> MGVALGATRVIYPAGQKQEQLAVTNNDENSTYLIQSWVENADGVKDGRFIVTPPLFAMKGKKE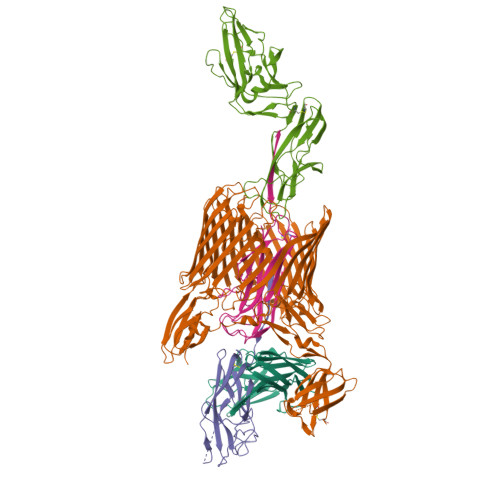NTLRILDATNNQLPQDRESLFWMNVKAIPSMDKSKLTENTLQLAIISRIKLYYRPAKLALPPDQAAEKLRFRRSANSLTLINPTPYYLTVTELNAGTRVLENALVPPMGESTVKLPSDAGSNITYRTINDYGALTPKMTGVME;> DLYFNPRFLADDPQAVADLSRFENGQELPPGTYRVDIYLNNGYMATRDVTFNTGDSEQGIVPCLTRAQLASMGLNTASVAGMNLLADDACVPLTTMVQDATAHLDVGQQRLNLTIPQAFMSNRARGYIPPELWDPGINAGLLNYNFSGNSVQNRIGGNSHYAYLNLQSGLNIGAWRLRDNTTWSYNSSDRSSGSKNKWQHINTWLERDIIPLRSRLTLGDGYTQGDIFDGINFRGAQLASDDNMLPDSQRGFAPVIHGIARGTAQVTIKQNGYDIYNSTVPPGPFTINDIYAAGNSGDLQVTIKEADGSTQIFTVPYSSVPLLQREGHTRYSITAGEYRSGNAQQEKPRFFQSTLLHGLPAGWTIYGGTQLADRYRAFNFGIGKNMGALGALSVDMTQANSTLPDDSQHDGQSVRFLYNKSLNESGTNIQLVGYRYSTSGYFNFADTTYSRMNGYNIETQDGVIQVKPKFTDYYNLAYNKRGKLQLTVTQQLGRTSTLYLSGSHQTYWGTSNVDEQFQAGLNTAFEDINWTLSYSLTKNAWQKGRDQMLALNVNIPFSHWLRSDSKSQWRHASASYSMSHDLNGRMTNLAGVYGTLLEDNNLSYSVQTGYAGGGDGNSGSTGYATLNYRGGYGNANIGYSHSDDIKQLYYGVSGGVLAHANGVTLGQPLNDTVVLVKAPGAKDAKVENQTGVRTDWRGYAVLPYATEYRENRVALDTNTLADNVDLDNAVANVVPTRGAIVRAEFKARVGIKLLMTLTHNNKPLPFGAMVTSESSQSSGIVADNGQVYLSGMPLAGKVQVKWGEEENAHCVANYQLPPESQQQLLTQLSAECRLVPRGSWSHPQFEK;> ADSTITIRGYVRDNGCSVAAESTNFTVDLMENAAKQFNNIGATTPVVPFRILLSPCGNAVSAVKVGFTGVADSHNANLLALENTVSAASGLGIQLLNEQQNQIPLNAPSSALSWTTLTPGKPNTLNFYARLMATQVPVTAGHINATATFTLEYQ;> ADVTITVNGKVVAKPCTVSTTNATVDLGDLYSFSLMSAGAASAWHDVALELTNCPVGTSRVTASFSGAADSTGYYKNQGTAQNIQLELQDDSGNTLNTGATKTVQVDDSSQSAHFPLQVRALTVNGGATQGTIQAVISITYTYS;> FACKTANGTAIPIGGGSANVYVNLAPVVNVGQNLVVDLSTQIFCHNDYPETITDYVTLQRGSAYGGVLSNFSGTVKYSGSSYPFPTTSETPRVVYNSRTDKPWPVALYLTPVSSAGGVAIKAGSLIAVLILRQTNNYNSDDFQFVWNIYANNDVVVPTGGCDVSARDVTVTLPDYPGSVPIPLTVYCAKSQNLGYYLSGTTADAGNSIFTNTASFSPAQGVGVQLTRNGTIIPANNTVSLGAVGTSAVSLGLTANYARTGGQVTAGNVQSIIGVTFVYQ>[3x]SHMTDDKKKGKFIVFEGLDRSGKSTQSKLLVEYLKNNNVEVKHLYFPNRETGIGQIISKYLKMENSMSNETIHLLFSANRWEHMNEIKSLLLKGIWVVCDR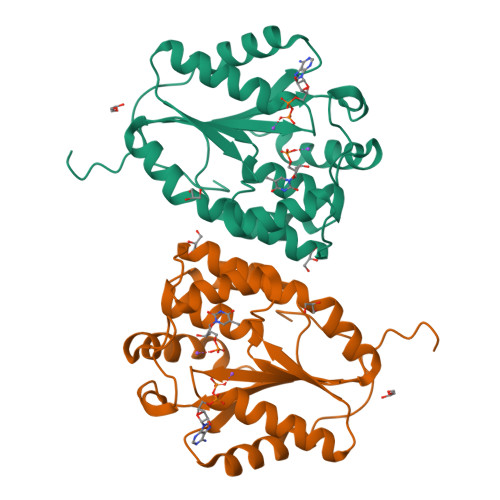YAYSGVAYSSGALNLNKTWCMNPDQGLIKPDVVFYLNVPPNYAQNRSDYGEEIYEKVETQKKIYETYKHFAHEDYWINIDATRKIEDIHNDIVKEVTKIKVEPEEFNFLWS> MQQQPPPDPAMRAALQSQPSGINSSDDWTQAMQRIMALTTRNPEAFRQQPQANRLSAILEAVVPSRSNPTHEKVLAIVNALVENKAIRGDEAGLVYNALLERVARYNSTNVQTNLDRMVTDVREAVAQRERFHRESNLGSMVALNAFLSTQPANVPRGQEDYTNFISALRLMVTEVPQSEVYQSGPDYFFQTSRQGLQTVNLSQAFKNLQGLWGVQAPVGDRATVSSLLTPNSRLLLLLVAPFTDSGSINRNSYLGYLINLYREAIGQAHVDEQTYQEITHVSRALGQDDPGNLEATLNFLLTNRSQKIPPQYTLSAEEERILRYVQQSVGLFLMQEGATPSAALDMTARNMEPSMYASNRPFINKLMDYLHRAAAMNSDYFTNAILNPHWLPPPGFYTGEYDMPDPNDGFLWDDVDSSVFSPRPGANERPLWKKEGSDRRPSSALSGREGAAAAVPEAASPFPSLPFSLNSIRSSELGRITRPRLLGEEEYLNDSLLRPEREKNFPNNGIESLVDKMSRWKTYAQEHRDDPSQGATSRGSAARKRRWHDRQRGL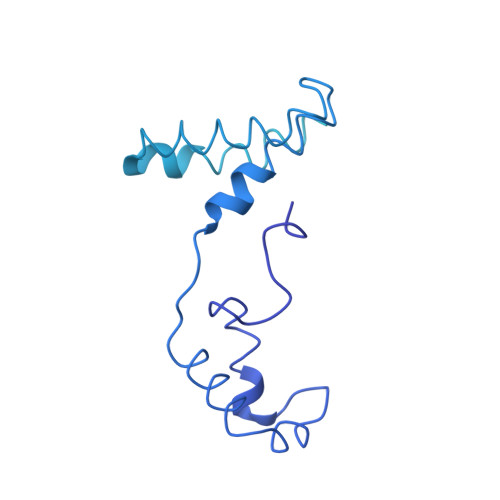MWDDEDSADDSSVLDLGGSGNPFAHLRPRIGRMM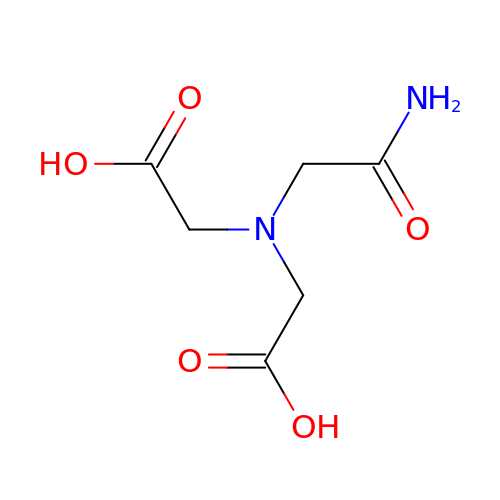(CARBAMOYLMETHYL-CARBOXYMETHYL-AMINO)-ACETIC ACID | C6 H10 N2 O5 | QZTKDVCDBIDYMD-UHFFFAOYSA-N>MSTKKKPTITKQELYSLVAADTQLNKALIERIFTSQQKIIQNALKHNQEVIIPPGIKFTVVTVKAKPARQGHNPATGEPIQIKAKPEHKAVKIR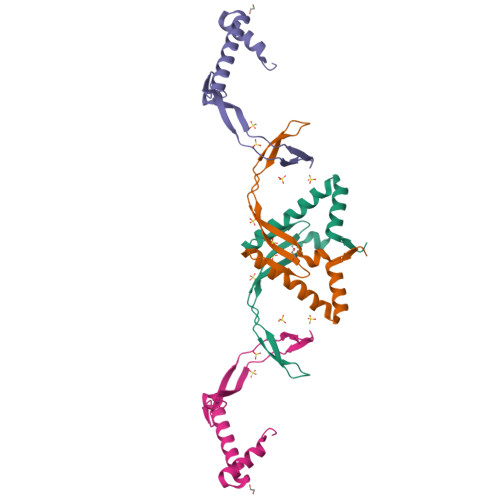ALKPVHDMLN[2x]> GSSQKFSTSPSPTLDDGLDRIKCPKKHGMKLLRAFPKLNDTAGGTSDYGWGFWCDRCHKEVPALI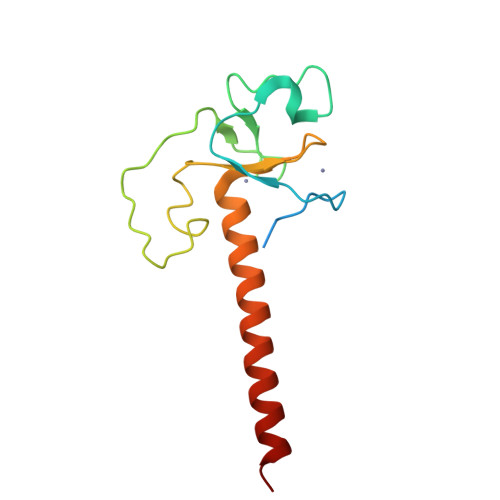KSKKRISKAQDERTHAPEENTFFYHCHCGYDLCKACGASIIHASNTLKENYSTELKNLAACFSTPS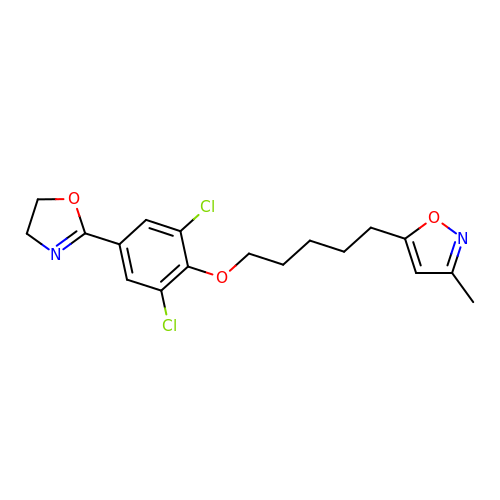5-(5-(2,6-DICHLORO-4-(4,5-DIHYDRO-2-OXAZOLY)PHENOXY)PENTYL)-3-METHYL ISOXAZOLE | C18 H20 Cl2 N2 O3 | JJDHAOLOHQTGMG-UHFFFAOYSA-N>[3x]MPEGPELHLASQFVNEACRALVFGGCVEKSSVSRNPEVPFESSAYRISASARGKELRLILSPLPGAQPQQEPLALVFRFGMSGSFQLVPREE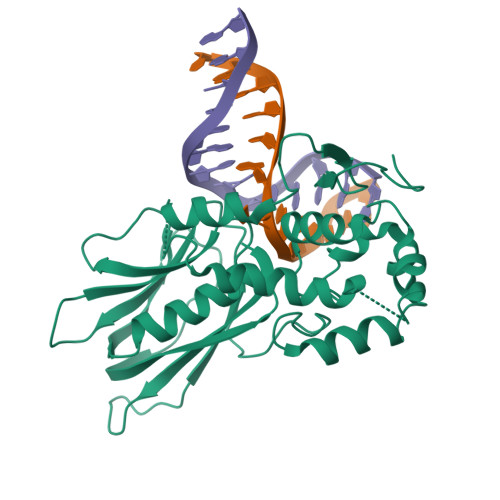LPRHAHLRFYTAPPGPRLALCFVDIRRFGRWDLGGKWQPGRGPCVLQEYQQFRENVLRNLADKAFDRPICEALLDQRFFNGIGNYLRAEILYRLKIPPFEKARSVLEALQQHRPSPELTLSQKIRTKLQNPDLLELCHSVPKEVVQLGGRGHGSESGEEDFAAFRAWLRCYGMPGMSSLQDRHGRTIWFQGDPGPLAPKGRKS> MSGKASTEGSVTTEFLSDIIGKTVNVKLASGLLYSGRLESIDGFMNVALSSATEHYESNNNKLLNKFNSDVFLRGTQVMYISEQ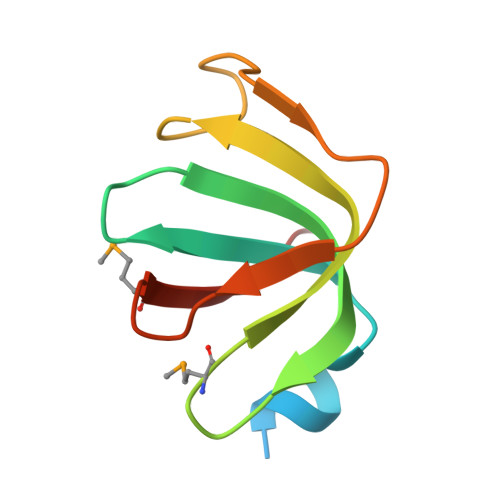KI> GSRFVVEKNNLKVTSPDSIKGIYECAIGNFGVPQYGGTLVGTVVYPKSNQKACKSYSD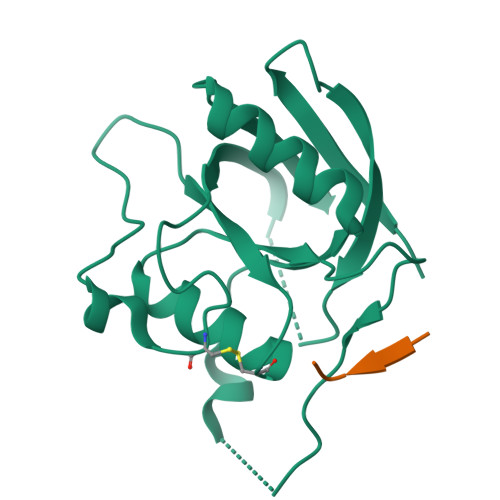FDISFKSKPGRLPTFVLIDRGDCYFTLKAWIAQQAGAAAILVADSKAEPLITMDTPEEDKSDADYLQNITIPSALITKTLGDSIKSALSGGDMVNMKLDWTESVPHP;> RVAAA N-{[1-methyl-4-(4-phenyl-1,3-thiazol-2-yl)piperidin-4-yl]methyl}-3-[5-(trifluoromethyl)-1,2,4-oxadiazol-3-yl]benzamide 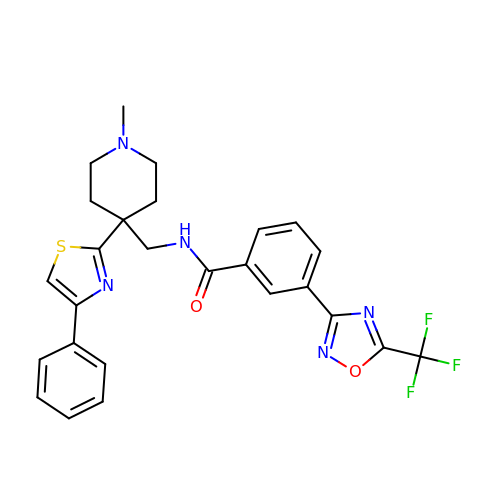| C26 H24 F3 N5 O2 S | BQFISAUAZNJOEG-UHFFFAOYSA-N NHLRC2 (NHL repeat containing protein 2) is an essential cytosolic protein of unknown function, mutation of which was recently identified in association with FINCA (fibrosis, neurodegeneration, cerebral angiomatosis) disease, a multi-organ condition which is fatal in early childhood. NHLRC2 contains three domains; an N-terminal thioredoxin-like (Trx-like) domain, followed by a six-bladed NHL repeat containing β-propeller domain and then a C-terminal β-stranded domain. The N-terminal Trx-like domain contains a CCINC motif at the position of the CXXC motif, which is characteristic of oxidoreductases and commonly involved in thiol-disulfide exchange. The six-bladed β-propeller domain comprises six NHL repeats, a structural motif originally identified in genes NCL-1, HT2A and LIN-41 and shown to often function as a protein-protein interaction module.

Crystals of the longer NHLRC2 fragment (aa 1–572) diffracted to 2.7 Å and also belong to space group P21 but contain four protein molecules in the asymmetric unit. However, in each molecule the electron density for first 9 amino acid residues, the loop connecting the Trx-like domain and β-propeller domain (212–219) and the fragment between residues 345 and 354 were either missing or of insufficient quality to allow the chain tracing, suggesting flexibility of these regions. As expected from the sequence analysis, the structure of the longer NHLRC2 fragment can be clearly separated into two domains. Consistent with this the Trx-like domain of NHLRC2 displays the common features of a thioredoxin fold, containing a central mixed β-sheet surrounded by three α-helices, along with a Trx8 family specific 26 amino acid insertion comprising an extra β-strand and 2 short α-helices inserted after the second β-strand of the thioredoxin-fold. There are also two additional N-terminal α-helices which fold over the Trx-like domain of NHLRC2 in the crystal structure, forming an N-terminal protrusion. The CXXC motif or CCINC in NHLRC2 (residues 89–93) is located at the N-terminus of α1 of the thioredoxin-fold, with Cys-89 and Cys-90 protruding from the protein surface. All cysteines of the CCINC motif are found in the reduced state.

>[4x]MHHHHHHMAAPGGRGRSLSGLLPAQTSLEYALLDAVTQQEKDSLVYQYLQKVDGWEQDLSVPEFPEGLEWLNTEEPISVYKDLCGKIVVLDFFTYCCINCIHLLPDLHALEHTYSDKDGLLIIGVHSAKFPNEKVLDNIKSAVLRYNITHPMVNDADASLWQELEVSCWPTLVILGPRGNMLFSLIGEGHKDKLFLYTSIALKYYKDRGQIRDNKIGIKLYKDSLPPSPLLFPGKVTVDQVTDRLVIADTGHHRILVVWKNGQIQYSIGGPNPGRKDGIFSESTFNSPQGVAIMNNIIYVADTENHLIRKIDLEAEKVSTVAGIGIQGTDKEGGAKGEQQPISSPWDVVFGTSGSEVQRGDILWIAMAGTHQIWALLLDSGKLPKKNELTKGTCLRFAGSGNEENRNNAYPHKAGFAQPSGLSLASEDPWSCLFVADSESSTVRTVSLKDGAVKHLVGGERDPMNLFAFGDVDGVGINAKLQHPLGVTWDKKRNLLYVADSYNHKIKVVDPKTKNCTTLAGTGDTNNVTSSSFTESTFNEPGGLCIGENGELLYVADTNNHQIKVMDLETKMVSVLPIF>GAMDPMICLGLEGTAEKTGVGIVTSDGEVLFNKTIMYKPPKQGINPREAADHHAETFPKLIKEAFEVVDKNEIDLIAFSQGPGLGPSLRVTATVARTLSLTLKKPIIGVNHCIAHIEIGKLTTEAEDPLTLYVSGGNTQVIAYVSKKYRVFGETLDIAVGNCLDQFARYVNLPHPGGPYIEELARKGKKLVDLPYTVKGMDIAFSGLLTAAMRAYDAGERLEDICYSLQEYAFSMLTEITERALAHTNKGEVMLVGGVAANNRLREMLKAMCEGQNVDF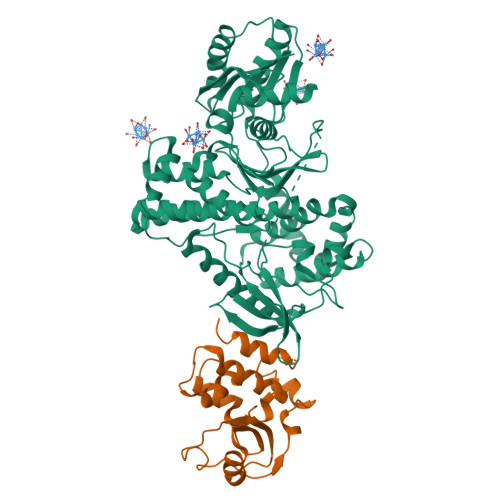YVPPKEFCGDNGAMIAWLGLLMHKNGRWMSLDETKIIPNYRTDMVEVNWIKEIKGKKRKIPEHLIGKGAEADIKRDSYLDFDVIIKERVKKGYRDERLDENIRKSRTAREARYLALVKDFGIPAPYIFDVDLDNKRIMMSYINGKLAKDVIEDNLDIAYKIGEIVGKLHKNDVIHNDLTTSNFIFDKDLYIIDFGLGKISNLDEDKAVDLIVFKKAVLSTHHEKFDEIWERFLEGYKSVYDRWEIILELMKDVERRARYVE[2x];>[2x]GAMDPMIIRGIRGARINNEIFNLGLKFQILNADVVATKKHVLHAINQAKTKKPIAKSFWMEILVRASGQRQIHEAIKIIGAKDGNVCLICEDEETFRKIYELIGGEIDDSVLEINEDKERLIREIFKIRGFGNVVERVLEKIALIELKKE> MLESNENRIQIMSTIAKIYRAMSRELNRRLGELNLSYLDFLVLRATSDGPKTMAYLANRYFVTQSAITASVDKLEEMGLVVRVRDREDRRAILIEITEKGLETFNKGIEIYKKLANEVTGDLSEDEVILVLD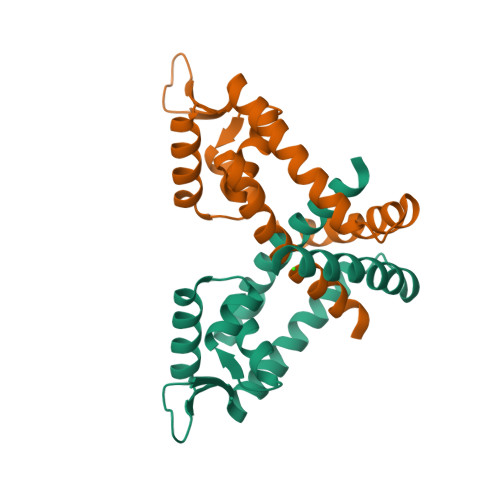KISKILKRIEEISQ> AAMEELQKSIGHKPEPTDEEWELIKTVTEAHVATNAQGSHWKQKQKFLPDDIGQAPIVNAPEGGKVDLEAFSHFTKIITPAITRVVDFAKKLPMFCELPCEDQIILLKGCCMEIMSLRAAVRYDPESETLTLNGEMAVTRGQLKNGGLGVVSDAIFDLGMSLSSFNLDDTEVALLQAVLLMSSDRPGLACVERIEKYQDSFLLA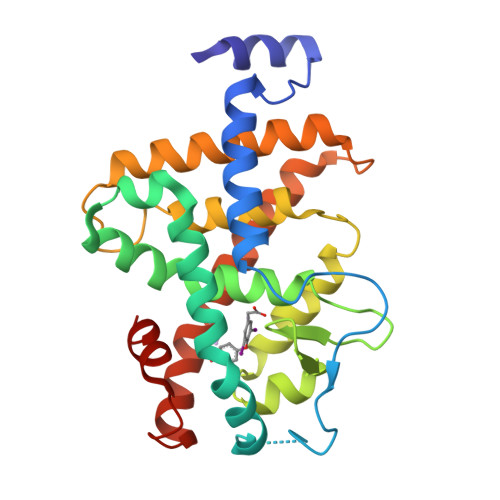FEHYINYRKHHVTHFWPKLLMKVTDLRMIGACHASRFLHMKVECPTELFPPLFLEVFED N,N-dimethyl-2-(4-phenoxyphenoxy)ethanamine 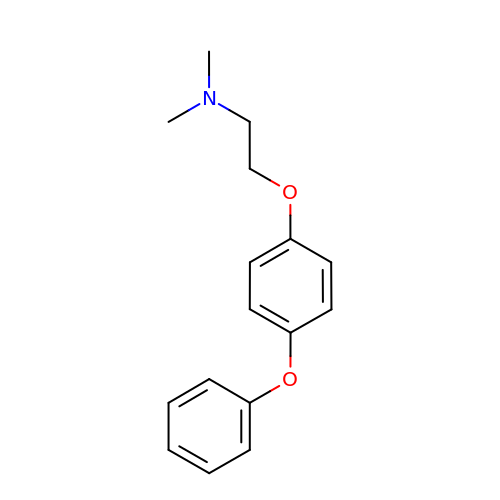| C16 H19 N O2 | INAQPAUETXGHJF-UHFFFAOYSA-N>YLQKPMYEVQWKVVEEINGNNYVYIDPTQLPYDHKWEFPRNRLSFGKTLGAGAFGKVVEATAYGLIKSDAAMTVAVKMLKPSAHLTEREALMSELKVLSYLGNHMNIVNLLGACTIGGPTLVITEYCCYGDLLNFLRRKRDSFICSKTSPAIMEDDELALDLEDLLSFSYQVAKGMAFLASKNCIHRDLAARNILLTHGRITKICDFGLARDIKNDSNYVVKGNARLPVKWMAPESIFNCVYTFESDVWSYGIFLWELFSLGSSPYPGMPVDSKFYKMIKEGFRMLSPEHAPAEMYDIMKTCWDADPLKRPTFKQIVQLIEKQISESTN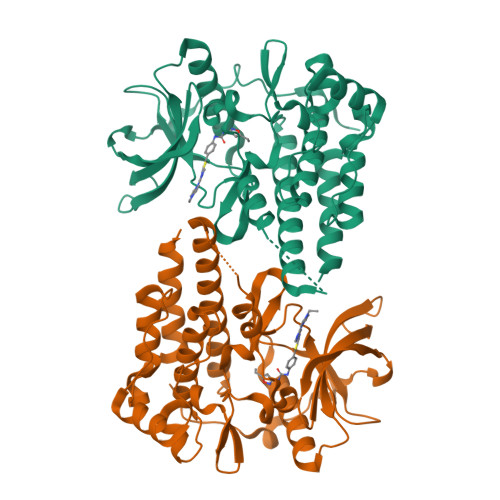HI[2x]>MLGLTLMFKRFFGAVRTSWRDPSTRGAVLSLAIIVTAATIFYTLAEKWSVIDSLFYAVSVGLPMGNGPLSPTLTLSKIFTLVYAILVVGLFVTVGGSLASAIVQNNTEKF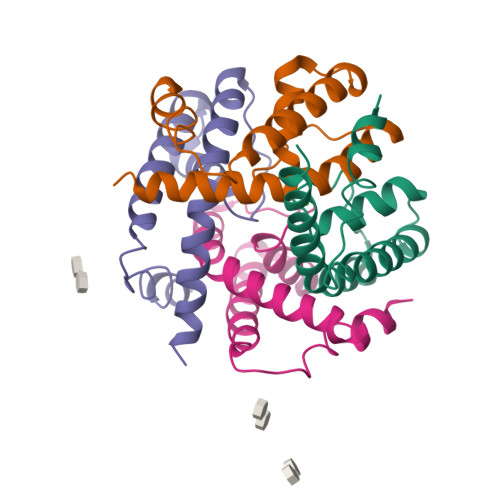KRLNRKGSAEAEDHHHHHH[6x]>[2x]GPLGSMGLAQEAHNVRVLGSGPQTVVLAHGFGTDQSVWKYLVPHLVEDYRVVLFDIMGAGTTNPTYFNFERYSSLEGYAGDVIAILEELQISSCVYVGHSVSAMIGVIASVTRPDLFTKLVTVAGSPRYLNDPDY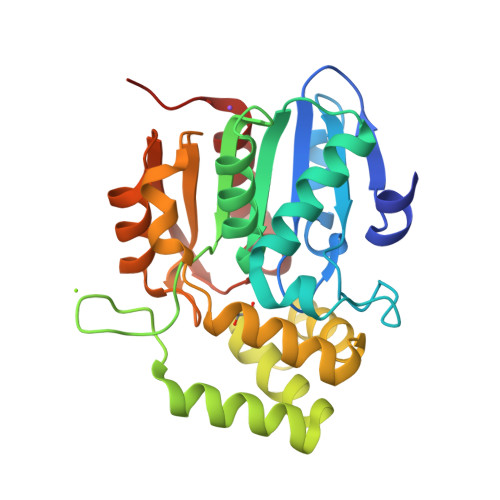FGGFDLDELHELFEAMKENYKAWCSGFAPLCVGADMESLAVQEFSRTLFNMRPDIALSILQTIFYSDVRPLLPHVTVPCHIIQSVKDLAVPVAVSEYIHQSLGGESILEVMATEGHLPQLSSPDVVVPVLLRHIRYAIARPN> GHMATGTRYAGKVVVVTGGGRGIGAGIVRAFVNSGARVVICDKDESGGRALEQELPGAVFILCDVTQEDDVKTLVSETIRRFGRLDCVVNNAGHHPPPQRPEETSAQGFRQLLELNLLGTYTLTKLALPYLRKSQGNVINISSLVGAIGQAQAVPYVATKGAVTAMTKALALDESPYGVRVNCISPGNIWTPLWEELAALMPDP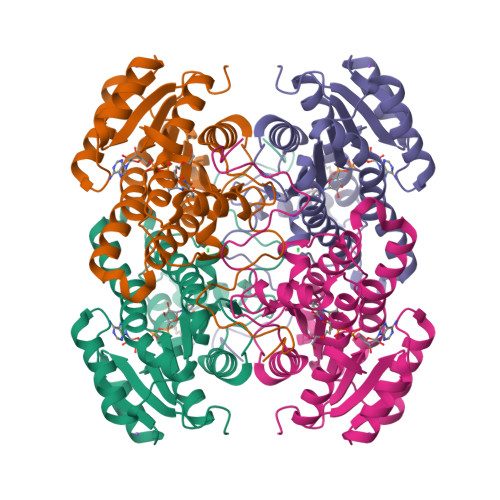RASIREGMLAQPLGRMGQPAEVGAAAVFLASEANFCTGIELLVTGGAELGYGCKASRSTPVDAPDIPSGS> ADADSLPHTKVTLVAPPQVHPHEQATASGPKVTEFTMTIEEKKMVIDDSGTTLQAMTFNGSMPGPTLVVHEGDYVQLTLVNPATNAMPHNVDFHGATGALGGAKLTNVNPGEQATLRFKADRSGTFVYHCAPSGMVPWHVVSGMSGTLMVLPRDGLKDPAGAPLHYDRAYTIGEFDLYIPKGPDGKYKDYATLAESYGDTVQVMRTLTPSHIVFNGKVGALTGANALTASVGETVLLIHSQANRDTRPHLIGGHGDWVWETGKFANPPQRDL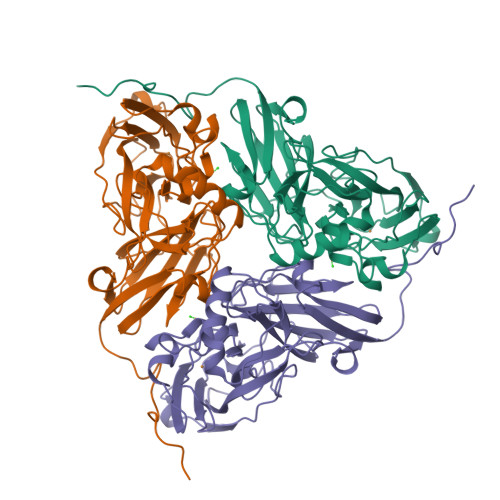ETWFIRGGSAGAALYTFKQPGVYAYLNHNLIEAFELGAAGHISVEGKWNDDLMKQIKAPAPIPA>[4x]SELYRQSLEIISRYLREQATGAKDTKPMGRSGATSRKALETLRRVGDGVQRNHETAFQGMLRKLDIKNEDDVKSLSRVMIHVFSDGVTNWGRIVTLISFGAFVAKHLKTINQESCIEPLAESITDVLVRTKRDWLVKQRGWDGFVEFFHVEDLEGG;>[4x]SENSLEIEELARFAVDEHNKKENALLEFVRVVKAKEQMGVNPEEMQTMYYLTLEAKDGGKKKLYEAKVWVKWWWGFHIWDNFKELQEFKPV

Pro‐apoptotic (or executioner) proteins such as BAK and BAX activate apoptosis through pore formation in the mitochondrial membrane; anti‐apoptotic proteins including BCL‐2, MCL‐1 and BCL‐xL, sequester pro‐apoptotic members to prevent cell death; and a group of regulatory proteins which bind to other BCL‐2 members (including BIM, BID, BAD, NOXA and PUMA), mediate initiation of apoptosis. In all cases binding between BCL‐2 family members occurs through the BH3 homology domain of one protein, which forms an α‐helix upon binding and docks into a complementary cleft on its partner. We have used phage display to isolate Affimer reagents (non‐antibody‐binding proteins based on a conserved scaffold) to identify ligands for MCL‐1, BCL‐xL, BCL‐2, BAK and BAX, then used multiple biophysical characterisation methods to probe the interactions. Co‐crystal structures reveal an unprecedented mode of molecular recognition; where a BH3 helix is normally bound, flexible loops from the Affimer dock into the BH3 binding cleft.

Similarly, the Affimers selected for MCL‐1 binding were shown to act as low μM inhibitors of their target interaction (MCL‐1‐AF1 IC50=2.1±0.2 μM; MCL‐1‐AF11 IC50=3.2±0.4 μM) but did not inhibit BCL‐xL /BAK,, demonstrating selectivity. Similarly, when comparing the structures of MCL‐1 bound to peptide versus Affimer we observe that the variable loops of the Affimer are inserted into the BH3 binding groove and that a desirable conformation is selected. In this case, the region where the protein conformation is affected is remote from the BH3 cleft, but again reflects a small molecule bound conformation. When BIM BH3 is bound, MCL‐1 adopts a nonhelical conformation at the QRN motif around Arg222. By contrast, when bound to Mule BH3 or a range of small molecules, the QRN motif is helical. Critically, when the QRN motif is helical, then ubiquitin can be added at this motif, and this promotes cellular degradation by the proteasome. Interestingly, our structure shows that MCL‐1‐AF11 also selects the desired helical, ubiquitylatable, conformation, again demonstrating that an Affimer can be isolated that selects a specific desired conformation. The helical QRN motif can be ubiquitylated; BH3 ligands that promote this conformation offer both orthosteric inhibition of BH3 binding and degradation by the proteasome to potentiate the removal of MCL‐1 function in cells. The Affimer again selects a conformation of a target protein to promote a desired functional outcome.> MNLSRRQLLALTSAGIAMGQASKLAAATKAAEQTGLKSAYKDNFLIGAALNATIASGADERLNTLIAKEFNSITPENCMKWGVLRDAQGQWNWKDADAFVAFGTKHNLHMVGHTLVWHSQIHDEVFKNADGSYISKAALQKKMEEHITTLAGRYKGKLAAWDVVNEAVGDDLKMRDSHWYKIMGDDFIYNAFTLANEV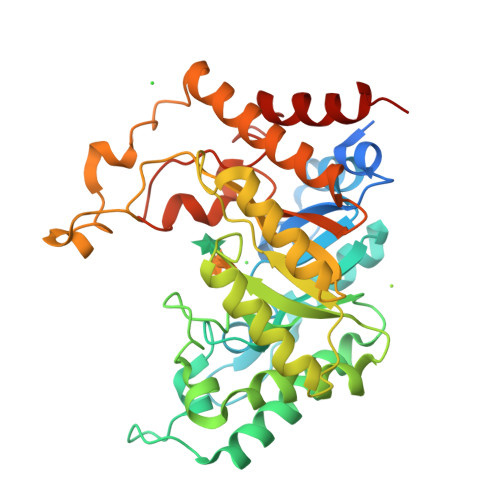DPKAHLMYNDYNIERTGKREATVEMIERLQKRGMPIHGLGIQGHLGIDTPPIAEIEKSIIAFAKLGLRVHFTSLDVDVLPSVWELPVAEVSTRFEYKPERDPYTKGLPQEMQDKLAKRYEDLFKLFIKHSDKIDRVTFWGVSDDASWLNDFSIPGRTNYPLLFDRKLQPKDAYFRLLDLKRLEHHHHH S-ADENOSYLMETHIONINE 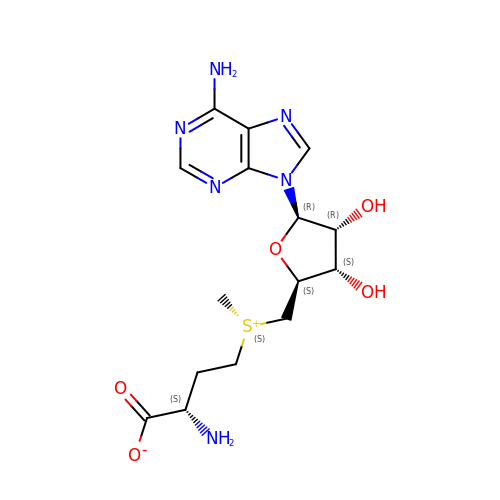| C15 H22 N6 O5 S | MEFKEPWMEQBLKI-FCKMPRQPSA-N DIGOXIGENIN | C23 H34 O5 | 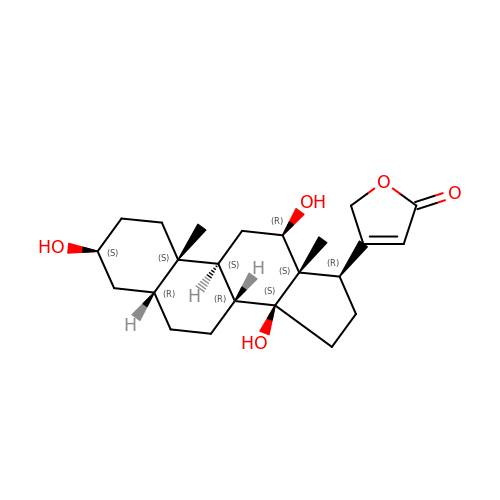SHIBSTMRCDJXLN-KCZCNTNESA-N> MSKKKFVIVSILTILLVQAIYFVEKYHTSEDKSTSNTSSTPPQTTLSTTKVLKIRYPDDGEWPGAPIDKDGDGNPEFYIEINLWNILNATGFAEMTYNLTSGVLHYVQQLDNIVLRDRSNWVHGYPEIFYGNKPWNANYATDGPIPLPSKVSNLTDFYLTISYKLEPKNGLPINFAIESWLTREAWRTTGINSDEQEVMIWIYYDGLQPAGSKVKEIVVPIIVNGTPVNATFEVWKANIG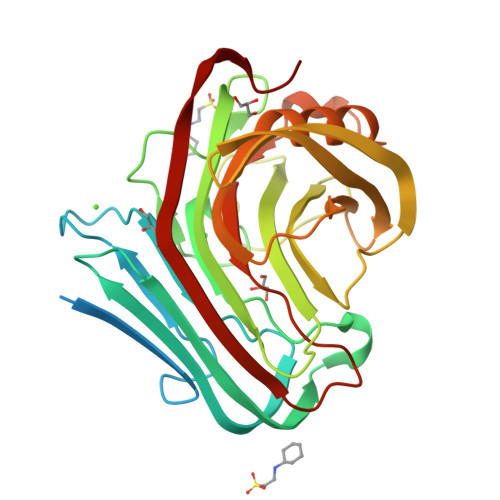WEYVAFRIKTPIKEGTVTIPYGAFISVAANISSLPNYTELYLEDVEIGTAFGTPSTTSAHLEWWITNITLTPLDRPLIS> MGRILDISGQPFDFDDEMQSRSDELAMVMKRTQEHPSSGVTPNRAAQMLRDAERGDLTAQADLAFDMEEKDTHLFSELSKRRLAIQALEWRIAPARDASAQEKKDADMLNEYLHDAAWFEDALFDAGDAILKGYSMQEIEWGWLGKMRVPVALHHRDPALFCANPDNLNELRLRDASYHGLELQPFGWFMHRAKSRTGYVGTNGLVRTLIWPFIFKNYSVRDFAEFLEIYGLPMRVGKYPTGSTNREKATLMQAVMDIGRRAGGIIPMGMTLDFQSAADGQSDPFMAMIGWAEKAISKAILGGTLTTEAGDKGARSLGEVHDEVRREIRNADVGQLARSINRDLIYPLLALNSDSTIDINRLPGIVFDTSEAGDITALSDAIPKLAAGMRIPVSWIQEKLHIPQPVGDEAVFTIQPVVPDNGSQKEAALSAEDIPQEDDIDRMGVSPEDWQRSVDPLLKPVIFSVL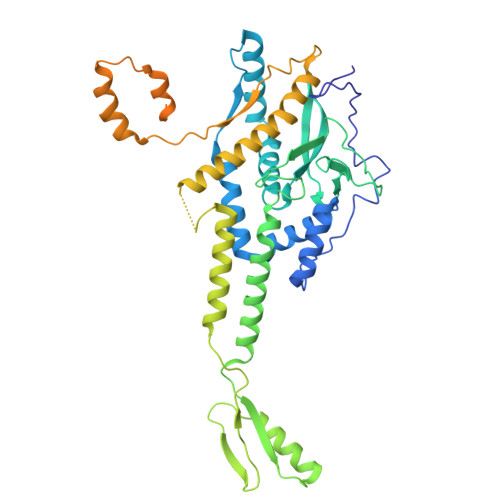KDGPEAAMNKAASLYPQMDDAELIDMLTRAIFVADIWGRLDAAADH5'-O-[(L-TRYPTOPHYLAMINO)SULFONYL]ADENOSINE | C21 H24 N8 O7 S | 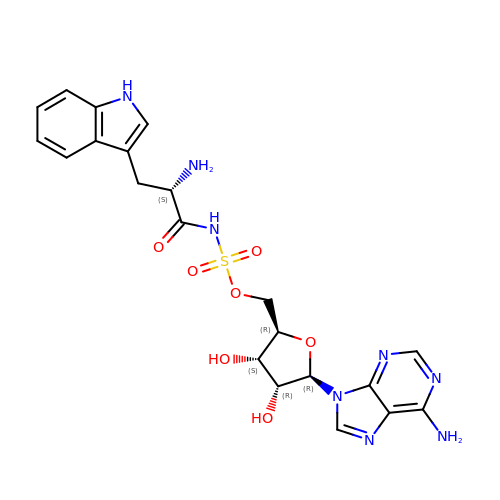RQAVKMXDGHWLGD-BFNSABJLSA-N>[2x]MNISPKAIKVRNIWIGGTEPC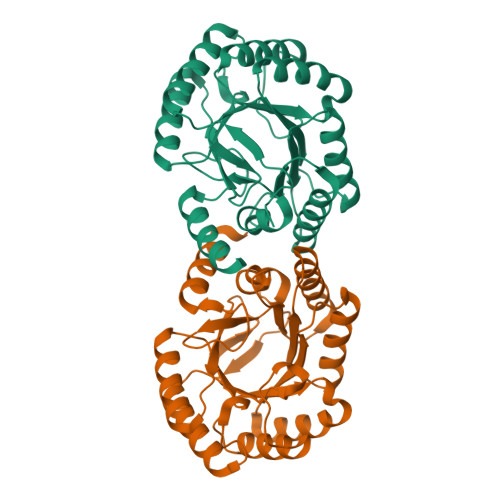ICAPVVGEDDRKVLREAEEVCRKQPDLLEWRADFFRAIDDQERVLATANGLRNIAGEIPILFTIRSEREGGQPIPLNEAEVRRLIEAICRSGAIDLVDYELAYGERIADVRRMTEECSVWLVVSRHYFDGTPRKETLLADMRQAERYGADIAKVAVMPKSPEDVLVLLQATEEARRELAIPLITMAMGGLGAITRLAGWLFGSAVTFAVGNQSSAPGQIPIDDVRTVLSILQTYSR4R-FLUORO-N6-ETHANIMIDOYL-L-LYSINE 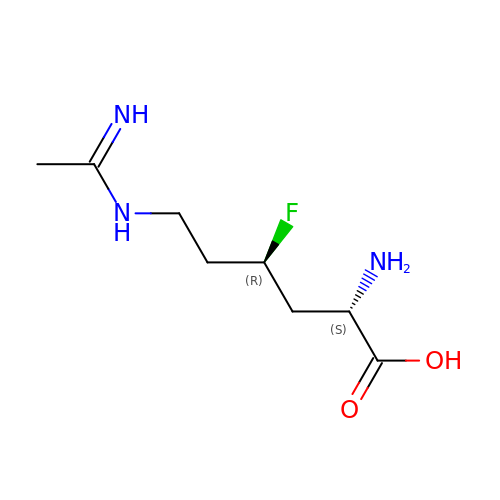| C8 H16 F N3 O2 | LTCJJIZTKXNFGK-RQJHMYQMSA-N> ETGQVAASPSINVALKAAFPSPPYLVELLETAASDNTTIYYSLLDRIAKGHFAEATTDKALYEKFLEVLRDDGHMDPEALSAFKLALSLRTATPRVEAHYQYYTATVEPSLSGTQEGCDQWFLIDGEQYCSPTLDTSHGKVKGEDQLRTLPFDRKFGVGSRDVILYADITSKSFAPFHEVAMDLAKKGKASYRVRYRRSPSHSRESLSVNGYGVELVLKRTDYIVIDDRDTGAAAKPAEENDQKPLVGHETVLDDGEEIADIKPLEKSELAALGMKAASFVMQSEKPFEALLKLTQDFPKYSNSLGSQNVSAEFEAEHRGNREVFLPEGSNVLWLNGLHLIDRQIQPFGLVDLLTRERKLIKSVLDLGLTGQQAVDLLGHAEVAHAKSGDDEPRRFDWRDDIEEGQVIIWLNNLEKDKRYKSFSPSIWVLIHHFGHGLPQIRRDVFNLVVPVDLTKADDVKIVVEGLLSFVKRLIPVRFGFVPLTPTGQAIDQAKVVYYLLENYGLAAATAYLEKSYEEQSTGQPNERIFNEVIKDKSLRPDGVELSFKDIFISEKHEKQIHLSKHWVERLRAGGDVPTVFFDGFPIPRECNWLRVMNHRLMQDLQALQQAGYFGMLNESMWLPGFFLEKALSRRNTLIFPEDKNELTVLNVNKIYIENHDLMSKVPVIEASKESTRDDWAALTVVADLDDIEGQELVYYALRFRKSNDGVRLDIVHNPKDTSRSPSVLAQRLKSREDKLLDFTRFLDLETALETGEFEPDVAYDASLANFLASSNMKAGDNFVILNGRVLGPITSADDFKKEDFEVFLQAERRTRILPVYKALEDLGLDDKVSGPLSAAKLTSVTALSTISDLPQGIFDNAPTVRTTLFKQWNSTYTSFEVGDASTATIFFVAVINPASEIGQRWVAVLKVLSELEGVHLRVFLNPTVMIEELPVKRFYRYVLSSSPSFDESGKVKALSARFTGVPRETLLVVGMDVPPAWLVTSKVAVDDLDNLRIKDI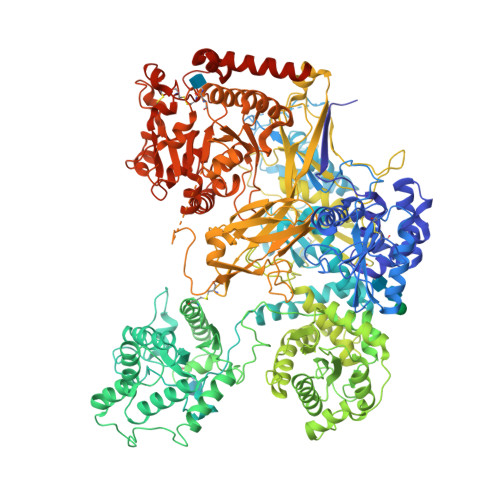KAKRGTEHVEAIYELEHILIEGHSREIPCAHAPRGVQLVLETENNPHFADTIIMANLGYFQFKANPGVYNIRLKEGRSSEIFTLESVGAKGWGPIPGDDNTEVVLMDFQGTTLYPRLRRKPGMEEEDVLEPSTKSGEESGSGARNLVSRGIKFAEGLLGRGNKAAEATKSVSKTEHAEINIFSVASGHLYERMLNIMMASVMHHTNHTVKFWFIEQFLSPSFKDFIPHMAAEYGFKYEMVTYKWPHWLRQQKEKQREIWGYKILFLDVLFPLSLDKVIFVDADQIVRTDMYDLVEHPLDGAPYGFAPMCDSRVEMEGYRFWKTGYWANYLKGKPYHISALYVVDLQRFRELAAGDRLRQQYHALSADPNSLANLDQDLPNHMQFTIPIATLPQEWLWCETWCSDETLKDARTIDLCNNPMTKEPKLDRARRQVPEWTKYDEEIAELARRVREEKPKKKEEEKVQKNPKSRRLDGDEEEVKTVREGTKHHHHHH2-azanyl-4-oxidanylidene-N-[(2S)-1-oxidanyl-3-phenyl-propan-2-yl]-3H-pteridine-7-carboxamide | 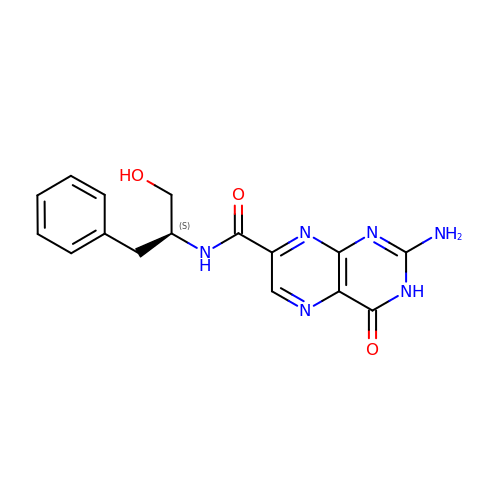C16 H16 N6 O3 | KWFPHGVJBSZTTG-JTQLQIEISA-N> MATIVDIAVNTPGFSTLVTAVKVANLVEALQSPGPFTVFAPNDDAFAKLPDGTITSLVQNPPQLGRI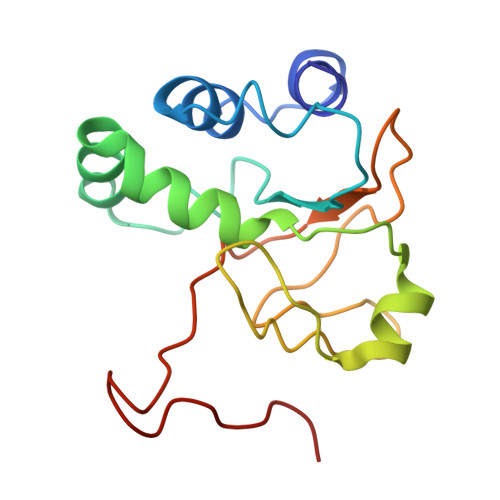LKYHVVAGAYKATDLKRMGIVTSLEGSTIPIHGDNPLEVKNATVLAADIEAENGIIHVIDTVILMGLDPAHSFQETNIPYKV>[2x]KPGAPWWKSAVFYQVYPRSFKDTNGDGIGDFKGLTEKLDYLKGLGIDAIWINPHYASPNTDNGYDISDYREVMKEYGTMEDFDRLMAELKKRGMRLMVDVVINHSSDQHEWFKSSRASKDNPYRDYYFWRDGKDGHEPNNYPSFFGGSAWEKDPVTGQYYLHYLGRQQPDLNWDTPKL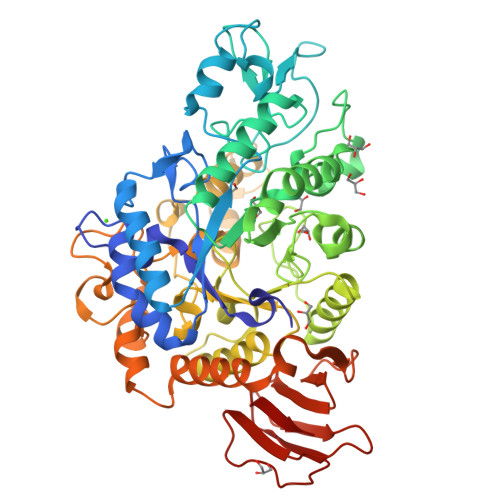REELYAMLRFWLDKGVSGMRFDTVATYSKTPGFPDLTPEQMKNFAEAYTQGPNLHRYLQEMHEKVFDHYDAVTAGEIFGAPLNQVPLFIDSRRKELDMAFTFDLIRYDRALDRWHTIPRTLADFRQTIDKVDAIAGEYGWNTFFLGNHDNPRAVSHFGDDRPQWREASAKALATVTLTQRGTPFIFQGDELGMTNYPFKTLQDFDDIEVKGFFQDYVETGKATAEELLTNVALTSRDNARTPFQWDDSANAGFTTGKPWLKVNPNYTEINAAREIGDPKSVYSFYRNLISIRHETPALSTGSYRDIDPSNADVYAYTRSQDGETYLVVVNFKAEPRSFTLPDGMHIAETLIESSSPAAPAAGAASLELQPWQSGIYKVK>HMAQDMRSEKRGLAYGYHSENDLKAMQGKVKWWYNWDTQADANVKENYASYGYDFVPMAWDENFNEEALRSFLDNHPDVKYLLGWNEPNFMEQANLTPAEAAAHWPVLEAIAQDYNLKLVAPAVNYSPGNVDIPGTDDDYDPWLYLDAFFEACEGCQVDYIAVHCYMKYESAFSWYVGEFERYNKPIWVTEWAGWDDGGPANMGEQMNFLSDTVRWMESNDNIYRYSWFLGRSSEGYDQFPYLDVLLADGELTPLGSVYTSIPSNDFRYKIPARIEAEGAHSLTGFKHLATTDTTGLAKLIAASNEVAEYKLNVEEGGDYTLALRLASSANSDIAIRVDGLLVYTFEDINTGGVEAWMTFSSTPISLTAGDHILRVESKSSRFGFNWLELTN[2x]

Our previous work revealed a curdlan-specific endo-β-1,3-glucanase, CBM6E, from a marine bacterium Saccharophagus degradans 2-40T, which contains an N-terminal GH128 module and a C-terminal CBM6 module. CBM6E exhibits catalytic activity at intermediate temperatures and efficiently produces GOS with DPs of 3–6 from curdlan. The CBM6 module of CBM6E (CBM6E-CBM6) exhibits a strong binding affinity specifically to curdlan, effectively enhancing the enzyme’s activity against curdlan. The GH128 and CBM6 modules form a cohesive structural entity, jointly recognizing triple-helical β-1,3-glucans.

The crystal structure of CBM6E was determined at a resolution of 2.4 Å. The structure of CBM6E comprises two distinct domains: an (α/β)-barrel catalytic domain (residues 84–348) belonging to the GH128 family, and a C-terminal β-sandwich domain (residues 349–473) belonging to the CBM6 family. The CBM6 domain forms an interdomain interface with GH128 primarily through hydrogen bonds between α8 and α9 of the GH128 domain and β10 and β13 of the CBM6 domain. Using the ConSurf web server, we identified that most of the residues at the interdomain interface are evolutionarily conserved. Notably, we observed a Mg2+ ion within CBM6E-CBM6, occupying a similar position as seen in ZgLamCCBM6. This ion demonstrated an six-coordinate octahedral geometry and coordinated with Glu357 OE1, Glu359 OE1, Ala379 O, Asn467 OD, Asn467 O, and a water molecule. To identify ancillary binding sites for curdlan triple helices, we conducted molecular docking experiments using a triple-helical β-1,3-glucan undecamer and the apo structure of CBM6E. In Model 1, the triple-helical β-1,3-glucan displayed a favorable structural complementarity with the CBM6 domain, while its nonreducing ends made contact with the GH128 domain. Model 2 revealed the triple-helical β-1,3-glucan spanning across the active groove of the GH128 domain. Overall, both docking models, in conjunction with the crystal structure of CBM6E in complex with GOS, support the hypothesis that triple-helical curdlan unwinding precedes its hydrolysis within the catalytic groove.>[4x]HMDKLPNIVILATGGTIAGSAATGTQTTGYKAGALGVDTL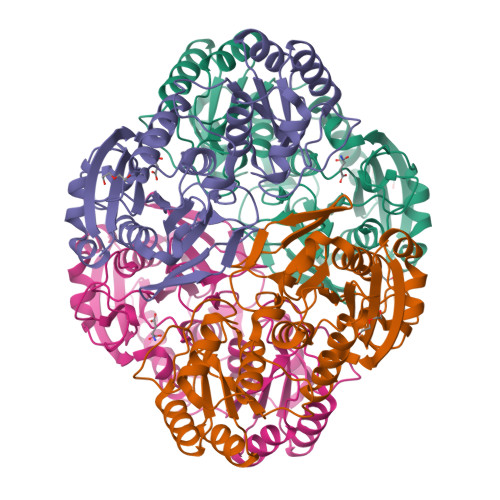INAVPEVKKLANVKGEQFSNMASENMTGDVVLKLSQRVNELLARDDVDGVVITHGTDTVEESAYFLHLTVKSDKPVVFVAAMRPATAISADGPMNLLEAVRVAGDKQSRGRGVMVVLNDRIGSARYITKTNASTLDTFKANEEGYLGVIIGNRIYYQNRIDKLHTTRSVFDVRGLTSLPKVDILYGYQDDPEYLYDAAIQHGVKGIVYAGMGAGSVSVRGIAGMRKAMEKGVVVIRSTRTGNGIVPPDEELPGLVSDSLNPAHARILLMLALTRTSDPKVIQEYFHTY Here we identified a novel transcription factor BswR, which is involved in the regulation of P. aeruginosa swarming motility and biofilm formation. No discernible motifs were found in both proteins, but bioinformatics analysis suggested that PA2780, comprising 114 amino acid residues, possesses a potential xenobiotic response element (XRE)-type DNA-binding domain at its N-terminus. Cumulatively, these results indicate that BswR positively regulates the transcriptional expression of the small RNA rsmZ by specifically binding to the promoter region of rsmZ. Further structural analyses suggest BswR functions as a homodimer, which uses positively charged helix to fit the major groove of the dsDNA for binding.

The crystal structure of BswR was determined and refined to 2.3 Å resolution. While 101 residues were visible in the final model, the last 13 residues and the 6×His-tag in C-terminus were not well ordered in the electron density map and thus excluded. The overall topology of BswR monomer contains seven helices, of which five form a compact helix bundle and the other two assemble as extended C-terminal helices. Consistent with the prediction, our structure reveals that the N-terminus of BswR comprises α2-turn-α3, a typical helix-turn-helix (HTH) motif for DNA-binding (in which α2 is for stabilization and α3 for recognition). Based on the gel filtration profile during protein purification, we found that BswR exists as a dimer in solution. This was further confirmed from the crystal structure: the two monomers with the V-shaped arrangement of the C-terminal helices intertwine together to form a homodimer by crystallographic symmetry. On dimerization, an average interface area of 1438.7 Å2 was buried, accounting for 20.8% of the solvent-exposed surface area (6923.4 Å2) of each monomer. Furthermore, dimerization was mainly mediated through hydrophobic interaction, which involves the residues Leu71, Leu74, Leu81, Phe85, Leu89, Thr90, Ile93, Leu97 and Ala99. In the dimeric structure, BswR exhibits an uncommon large area of dimer interface, which is formed by the extension of C-terminal helical region (helices 5–7, residues 61–101). In particular, BswR shares the most similar structure to C protein Csp231I, with a root-mean-square deviation (rmsd) of 1.169 Å for the main chain.

> MLGTRLKAARIRAGYSQKQLGMLVGMDEFSASARMNQYERERHSPNMRTSEQLAMVLQVPMAYLYCPEDELAELILKVSSLTPEFKKELTRFIEQLLAAQGSTSRQPVRTRSELLEHHHHHH> MQKNPISPTIPLDRDGVFHGFLKLPHSRDDSAWGSVMIPLTVIKNGAGPTALLTGANHGDEYEGPVALHELAATTSAEDVTGRLIIVPAFNYPAFRAGSRTSPIDRGNLNRSFPGRPDGTVTEK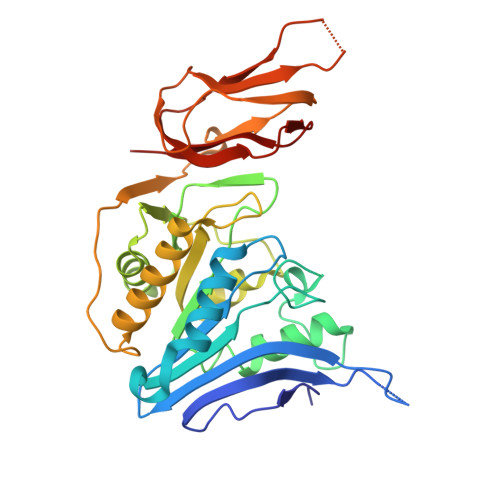IADYFQRTLLPMADLAVDFHSGGKTLDFVPFAAAHILDDKATQAACFAAMKAFNAPYSVELLEIDSAGMYDTAVEEMGKVLVTTELGGGGSSSARSNAIAKKGLRNVLIHAGILKGEMQLDETVNLTMPDDDCFVFSEGDGLFEMMIDLGAPVAKGDLLARVWPLDRTGQPPVEYRARRAGLVISRHFPGLIKSGDCVAVVGVTGA> WGSGEVKQKLQEFLL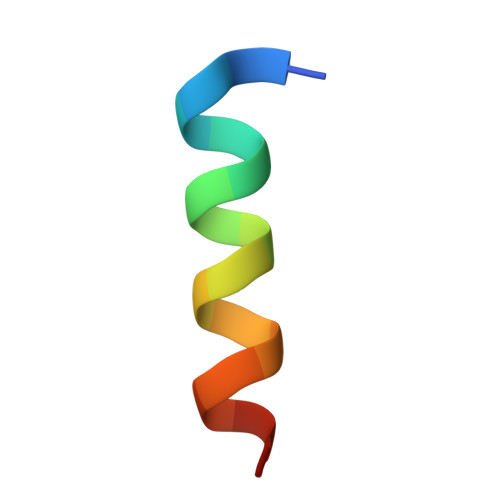SKS Peptidyl-prolyl isomerases (PPIases) catalyze cis/trans isomerization of peptidyl-prolyl bonds, which is often rate-limiting for protein folding. SlyD is a two-domain enzyme containing both a PPIase FK506-binding protein (FKBP) domain and an insert-in-flap (IF) chaperone domain. In order to improve our understanding of the mechanism of SlyD and of FKBPs in general, we set out to analyze the kinetics, energetics, and structural basis for substrate binding and inhibition of SlyD from Thermus thermophilus (TtSlyD) using 15-residue-long unmodified peptides, which we reasoned would be better mimics of natural unfolded protein substrates than the traditionally used 4-nitroanilide tetrapeptides. In total, we obtained five structures of TtSlyDFL and three of TtSlyDΔIF at a maximum resolution of up to 1.4 Å.

Next, we tested binding of an S2 mutant peptide where the sole tryptophan residue was replaced by alanine (S2-W23A). This peptide retained the ability to bind to both domains of TtSlyDFL, albeit with moderately reduced affinities. Furthermore, there is more than one molecule of TtSlyD in the asymmetric unit in several cases, which for TtSlyDFL:S2 and TtSlyDFL:S2-W23A display substantial differences in substrate binding. We therefore expected that a peptide where W23S2 is mutated to alanine would bind similarly to the S2 peptide bound to molecule B in the TtSlyDFL:S2 structure. Surprisingly, the structure of TtSlyDFL:S2-W23A revealed instead a third binding mode where F30S2 and I31S2 are inserted into the binding groove. The S2 and S2-W23A peptides both bind by inserting the side chain of P29S2 in cis form into the center of the binding pocket. The binding mode is the same for both TtSlyDFL molecules in the TtSlyDFL:S2 structure, whereas the S2-W23A peptide binds in two different ways to the four molecules in the TtSlyDFL:S2-W23A structure: one similar to the S2 peptide (molecules A and C), and one in a different but partially overlapping fashion (molecules B and D). Two peptides, S2 and S2-W23A, adopt β-turn structures with a cis-proline in the i + 2 positions. However, our results speak against such a scenario, because both type VIa1 and distorted VIb β-turns are observed in our TtSlyDFL:S2, TtSlyDFL:S2-W23A, and TtSlyDΔIF:S2-W23A structures, which strongly suggests that FKBPs can catalyze cis/trans isomerization of prolines present in (at least) both these two types of β-turns.

>[4x]MKVGQDKVVTIRYTLQVEGEVLDQGELSYLHGHRNLIPGLEEALEGREEGEAFQAHVPAEKAYGPHDPEGVQVVPLSAFPEDAEVVPGAQFYAQDMEGNPMPLTVVAVEGEEVTVDFNHPLAGKDLDFQVEVVKVREATPEELLHGHAHLVPK;>TRYANPKMKPFIFGAX[9x]>GSHMNIMYDMISDLNERSEDFE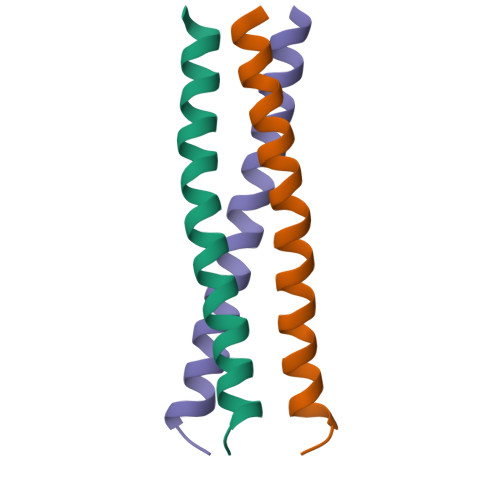KRIVTLETKLETLIGSIHALP[2x]>FQGAMDPEFSMKIGIIGAMEEEVTLLRDKIENRQTISLGGCEIYTGQLNGTEVALLKSGIGKVAAALGATLLLEHCKPDVIINTGSAGGLAPTLKVGDIVVSDEARYHDADVTAFGYEYGQLPGCPA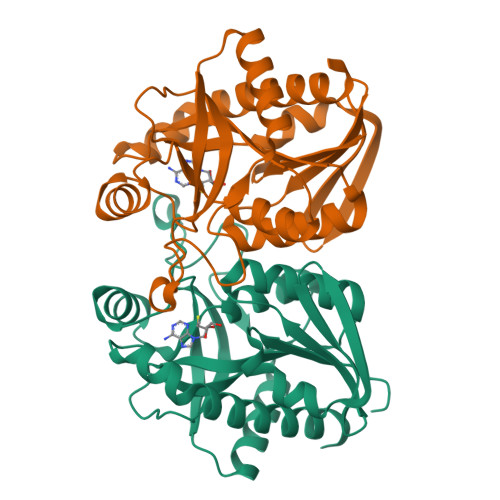GFKADDKLIAAAEACIAELNLNAVRGLIVSGDAFINGSVGLAKIRHNFPQAIAVEMEATAIAHVCHNFNVPFVVVRAISNVADQQSHLSFDEFLAVAAKQSSLMVESLVQKLAHG[2x]> TFSYTLEDHTKQAFGIMNELRLSQQLCDVTLQVKYQDAPAAQFMAHKVVLASSSPVFKAMFTNGLREQGMEVVSIEGIHP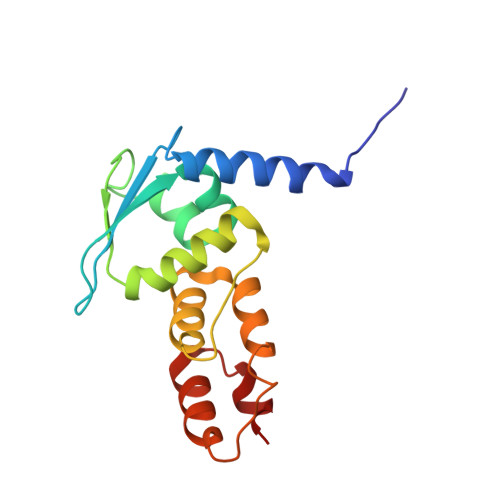KVMERLIEFAYTASISMGEKCVLHVMNGAVMYQIDSVVRACSDFLVQQLDPSNAIGIANFAEQIGCVELHQRAR>ASDDNVFQPVDQLPEDLIPSSIQVLKFSGKYLKLEQDKAYFDWPGFKTAIDNYTGEDLSFDKYDQSTINQQSQEVGAMVDKIAKFLHDAFAAVVDLSKLAAIILNTFTNLEEESSSGFLQFNTNNVKKNSSWEYRVLFSVPFGDNAPSYFYSLVTTILITADIEEKTGWWGLTSSTKKNFAVQIDALEL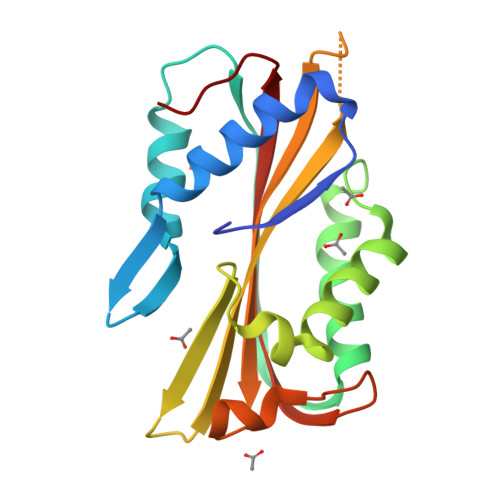VVKKGFKAPN[4x]>[2x]MTNLPTALITGASSGIGATYAERFARRGHNLVMVARDKVRMDVLASRLREETKVTIDVIQADLTQQKDLAEVETRLREDTSIGILINNAGMGQSGAFVQQNAQSIDRLVMLNTTAPTRLAAAVAARFAQEGKGSIVNIGSVVGFAPELGMTIYGATKAFVLFLSQGLNLELGPKGIYV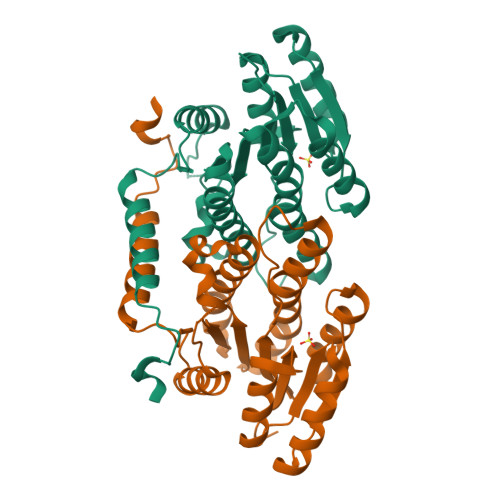QAVLPAATRTEIWSRAGMDINTLPEVMDVNELVDAALIGFDRKELVTIPPLHVAERWNELDQARQGLMSEIRQAHAAERYLPQALEHHHHHH> SPIPVTVREHKGCFYSTNPDTTVPIYGKTISTPSDYMCGEFSDLLELCKLPTFLGNPNTNNKRYPYFSATNSVPATSMVDYQVALSCSCMANSMLAAVARNFNQYRGSLNFLFVFTGAAMVKGKFLIAYTPPGAGKPT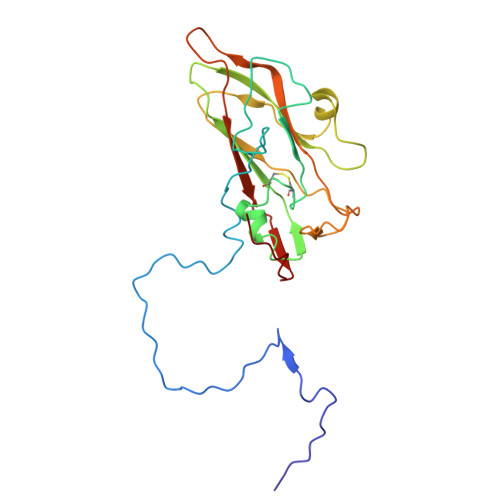TRDQAMQSTYAIWDLGLNSSFNFTAPFISPTHYRQTSYTSPTITSVDGWVTVWQLTPLTYPSGTPTNSDILTLVSAGDDFTLRMPISPTKWVPQ Mycobacterium tuberculosis (Mtb) WhiB3 is an iron–sulfur cluster-containing transcription factor belonging to a subclass of the WhiB-Like (Wbl) family that is widely distributed in the phylum Actinobacteria. WhiB3 plays a crucial role in the survival and pathogenesis of Mtb. It binds to the conserved region 4 of the principal sigma factor (σA4) in the RNA polymerase holoenzyme to regulate gene expression like other known Wbl proteins in Mtb. Here we determined crystal structures of the WhiB3:σA4 complex without and with DNA at 1.5 Å and 2.45 Å, respectively, to elucidate how WhiB3 interacts with DNA to regulate gene expression. These structures reveal that the WhiB3:σA4 complex shares a molecular interface similar to other structurally characterized Wbl proteins and also possesses a subclass-specific Arg-rich DNA-binding motif.

We then cocrystallized the WhiB3:σA4-βtip complex with PwhiB7 that was used in the crystallographic study of the WhiB7:σA4-βtip:PwhiB7 complex, which enabled us to collect high-quality diffraction data from a WhiB3:σA4-βtip:PwhiB7 crystal and refined the crystal structure at 2.45-Å resolution with the final Rfree/Rwork value of 0.211/0.243 (see Experimental procedures). A structural comparison shows that although both WhiB3 and σA4 in the WhiB3:σA4-βtip:PwhiB7 structure are involved in DNA binding like the case of WhiB7, they are dramatically different in how the Wbl-bound σA4 interacts with PwhiB7. σA4 of the WhiB3:σA4 complex orients about 180° relative to the WhiB7-bound σA4 along with the PwhiB7 DNA and inserts into the major groove upstream of the AT-rich WhiB7 binding site instead of the expected −35 element. Therefore, the observation that σA4 in the WhiB3:σA4-βtip:PwhiB7 complex binds to a physiologically irrelevant site of PwhiB7 opposite to the direction of transcription initiation indicates that PwhiB7 is unlikely a target of WhiB3. However, the crystal structure of the WhiB3:σA4-βtip:PwhiB7 complex provides valuable insights into the general features of how WhiB3 interacts with DNA, which is the primary focus of our structural analysis below. Although a “RGR” sequence is also present in the Arg-rich motif (“RGRAR”) of Mtb WhiB3, the RGR sequence is not conserved in the WhiB3 subclass and only R38 in the motif inserts vertically into the minor groove of the junction between the WhiB7 binding site and the −35 element. R38 forms polar contacts with the nucleotides of 2 GC pairs, in contrast to the preference of AT-rich DNA by the WhiB7 AT-hook. The other conserved residue in the Arg-rich motif, R42, is near the edge of the DNA duplex (∼4 Å away) and thus may form hydrophilic interactions with the phosphate backbone in solution. The central minor-groove width (∼3.5 Å) around the AT-rich region of PwhiB7 in WhiB3:σA4-βtip:PwhiB7 is characteristic of A-track DNAs and is significantly narrower than that of WhiB7:σA4-βtip:PwhiB7 (∼7 Å) where WhiB7-bound to the minor groove of the AT-rich region.

> MPQPEQLPGPNADIWNWQLQGLCRGMDSSMFFHPDGERGRARTQREQRAKEMCRRCPVIEACRSHALEVGEPYGVWGGLSESERDLLLKGTMGRTRGIRRTA;> MAHHHHHHVAVDAVSFTLLQDQLQSVLDTLSEREAGVVRLRFGLTDGQPRTLDEIGQVYGVTRERIRQIESKTMSKLRHPSRSQVLRDYLDGSSGSGTPEERLLRAIFGEKA>MRGSHHHHHHGLVPRGSMKITVLGCGALGQLWLTALCKQGHEVQGWLRVPQPYCSVNLVETDGSIFNESLTANDPDFLATSDLLLVTLKAWQVSDAVKSLASTLPVTTPILLIHNGMGTIEELQNIQQPLLMGTTTHAARRDGNVIIHVANGITHIGPARQQDGDYSYLADILQTVLPDVAWHNNIRAELWRKLAVNCVINPLTAIWNCPNGELRHH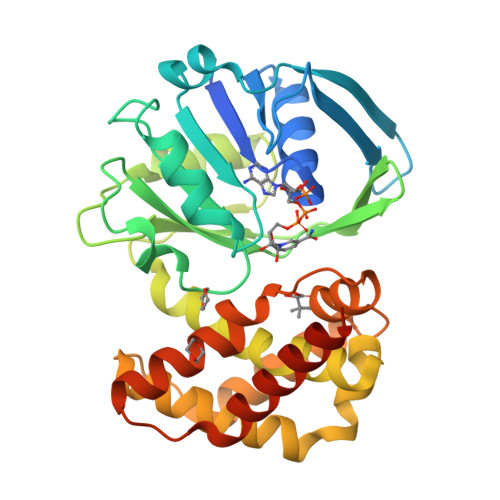PQEIMQICEEVAAVIEREGHHTSAEDLRDYVMQVIDATAENISSMLQDIRALRHTEIDYINGFLLRRARAHGIAVPENTRLFEMVKRKESEYERIGTGLPRPW[2x]>[2x]SMTATLRDAVAADLRSITEIYRESVLNGVATYEETPPSEAEMALRFSTITGNGYPYVVALDERGAVIGYAYASAFRNRTAYRFLVEDSIYLSPEARGKGIGKA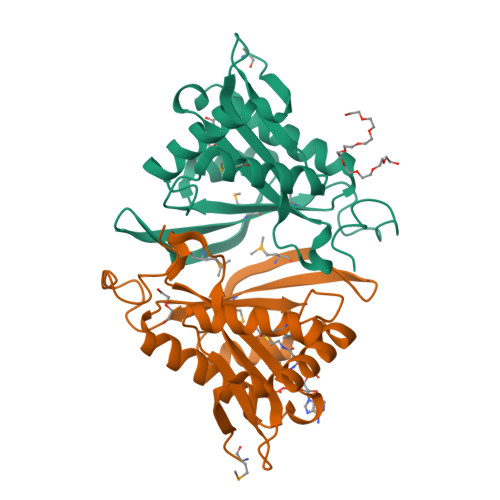LLSELVGRCTALGFRQMIAVIGGAHPSSIALHRALGFELQGLMKATGFKHGRWLDTAFMQRPLGEGTATKPTEGVYPDTLYRS> MGHHHHHHSGIALSRLAQERRAWRKDHPFGFVAVPTKNPDGTMNLMNWECAIPGKKGTPWEGGLFKLRMLFKDDYPSSPPKCKF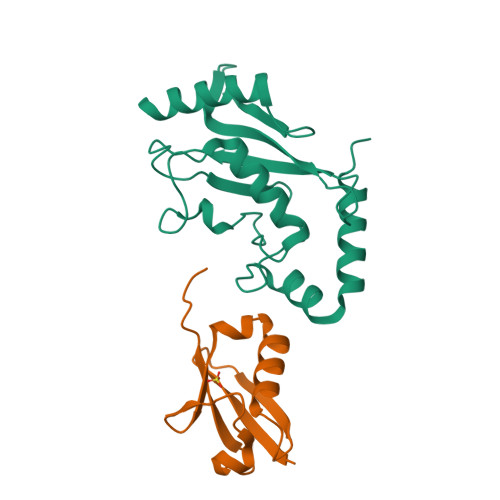EPPLFHPNVYPSGTVCLSILEEDKDWRPAITIKQILLGIQELLNEPNIQDPKQAEAYTIYCQNRVEYEKRVRAQAKKFAPS;> MGSSHHHHHHEGEYIKLKVIGQDSSEIHFKVKMTTHLKKLKESYCQRQGVPMNSLRFLFEGQRIADNHTPKELGMEEEDVIEVYQEQTGG methyl 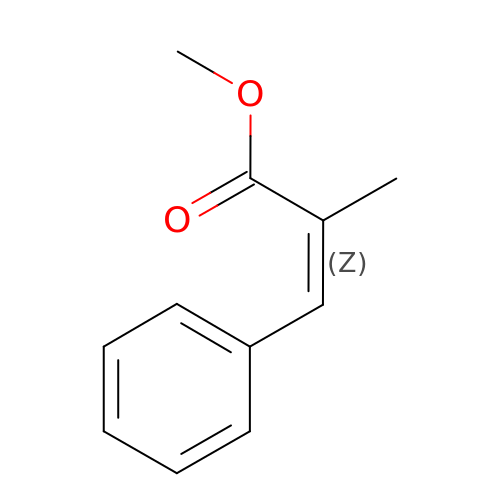(~{Z})-2-methyl-3-phenyl-prop-2-enoate | C11 H12 O2 | QILOUBBQVGUFNG-HJWRWDBZSA-N(4-{6-[(2S)-4-(2,4-diamino-6-ethylpyrimidin-5-yl)but-3-yn-2-yl]-2H-1,3-benzodioxol-4-yl}phenyl)acetic 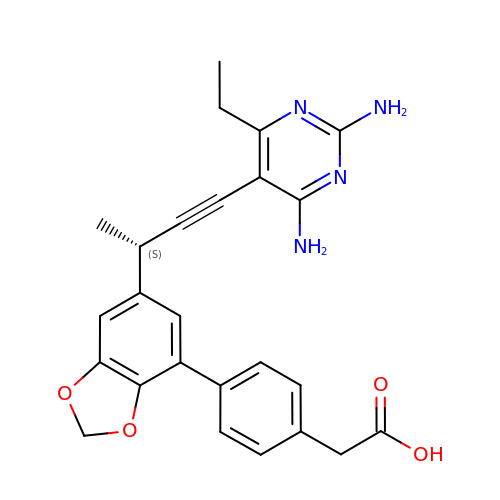acid | C25 H24 N4 O4 | DFNOGZMANMBRCF-CQSZACIVSA-N> MKLPVAQYSAPD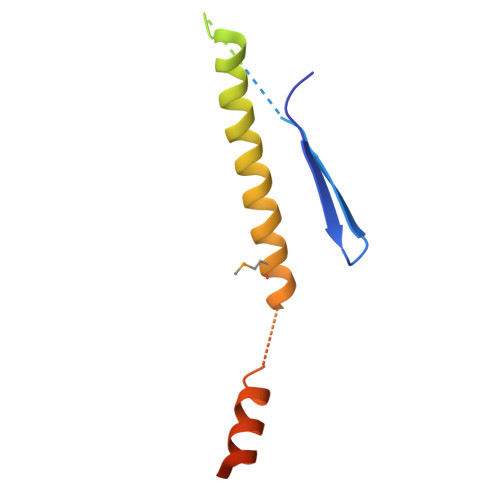GVEKSFAPIRDDPRYMTTEGRTTGPSDHVLNAGQIDRDKPSEPERTKDGSQLTYLGQLRTQLTGLQDDINEFLTGRMELAKNKKKAGADEKRIQEEINQLLDGGDGDEDAV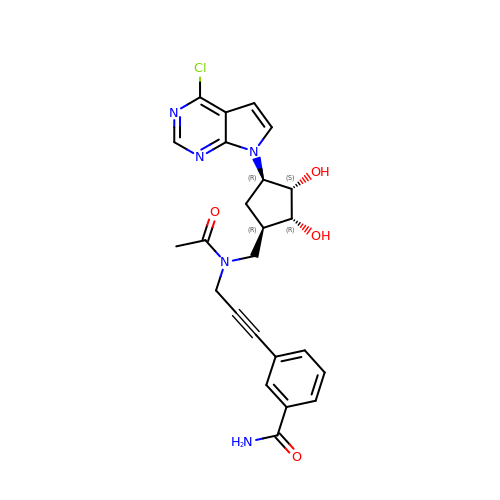3-[3-(acetyl{[(1R,2R,3S,4R)-4-(4-chloro-7H-pyrrolo[2,3-d]pyrimidin-7-yl)-2,3-dihydroxycyclopentyl]methyl}amino)prop-1-yn-1-yl]benzamide | C24 H24 Cl N5 O4 | AHVJTPYPUIHNLS-WLRLJWMZSA-N Here we report a saponin acetyltransferase from Astragalus membranaceus. AmAT7-3 is discovered through a stepwise gene mining approach and characterized as the xylose C3′/C4′-O-acetyltransferse of astragaloside IV. AmAT7-3 is a rare multi-site acetyltransferase which acetylate large saponin molecules. We solved the crystal structures of AmAT7-3 and its variant A310G in complex with astragaloside IV, respectively.

The variants A310G and A310W were found to catalyze specific C3′-O and C4′-O acetylation for astragaloside IV, respectively. A310D/G/R selectively catalyzed the C3′-OH acetylation of 1, while A310F/W specifically favored C4′-OH. MD simulations showed that the substrate binding is relatively stable in both AmAT7-3A310G and AmAT7-3A310W, with only one major conformation. In the A310G variant, as the steric hindrance of the methyl group is removed from Ala, L290 was able to move closer to G310, leading to a simultaneous rotation of the sugar ring towards L290. As a result, the sugar ring in AmAT7-3A310G rotated counterclockwise by 80° compared to that in the wild-type, while in A310W it rotated clockwise by 30°. For A310G, O3 was almost perpendicular (92.9°) to the plane where the C = O group is located, while O4 formed an angle of 47.8° with C = O plane. The vertical position was more favorable for the nucleophilic attack reaction. As a result, the O3- acetylation was kinetically favored over the O4- acetylation in AmAT7-3A310G, which was consistent with the biochemical experimental results. QM/MM calculations showed that the energy barrier of the first reaction step was 19.9 kcal/mol for the O3-acetylation and 30.0 kcal/mol for the O4-acetylation, respectively. The A310G variant catalyzed 5 to generate a single product with a conversion rate of 96.3%.

> MSSLRLVSSSTIQAANDNNDDSSQLIDLTVWDLIGLERESIQQGLLYHHPNQVDTPNQIQHLKHSLSSTLSFFPPFAGRLVITEYEDNTATCFIACNNAGALFVHAVAENTTISDILQPNKYVPPIVNSLFSLNGVKNREGTIQPLLVVQVTELVDGIFIGLTVNHVVADGKSFWLFVNSWAEISRGFQKPSKLPTLERWFLNDTDHPIRFSFSMEEEKKKFQSGQLTTRFFHFTRENIAHLKSKANGEVTLGNTERRISSLQALLAHVWRSVVRCERIDPQEVLYYILLIDARTRLIPPLEDDYFGNAGDAGVVIMKAGELLEGGLGNVAWNMNKVISLNSDEKIKNRYKSWLRTPQLPSMGMHTTFASQLLIIANSPRFNVYGNDFGWGKPLAVRSSAENKRDCKIVLFAGAEEGSIDIEVCLPYEILEALGNDAEFLDNHSIG>[2x]AIRNCIIGKGRSYKGTVSITKSGIKCQPWSSMIPHEHSFLPSSYRGKDLQENYCRNPRGEEGGPWCFTSNPEVRYEVC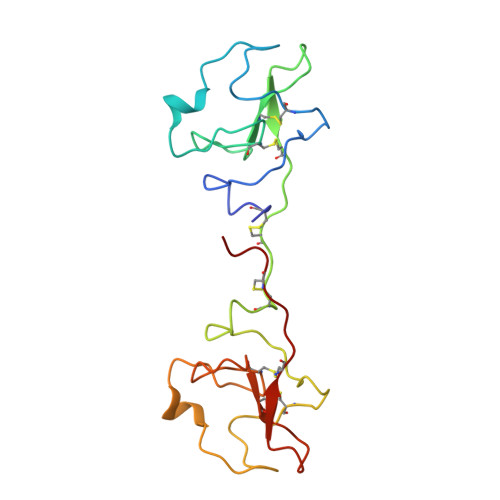DIPQCSEVECIIGKGRSYKGTVSITKSGIKCQPWSSMIPHEHSFLPSSYRGKDLQENYCRNPRGEEGGPWCFTSNPEVRYEVCDIPQCSEVE>MSPLSGSLAPLNMKGLVKFQDVSFAYPNHPNVQVLQGLTFTLYPGKVTALVGPNGSGKSTVAALLQNLYQPTGGKVLLDGEPLVQYDHHYLHTQVAAVGQEPLL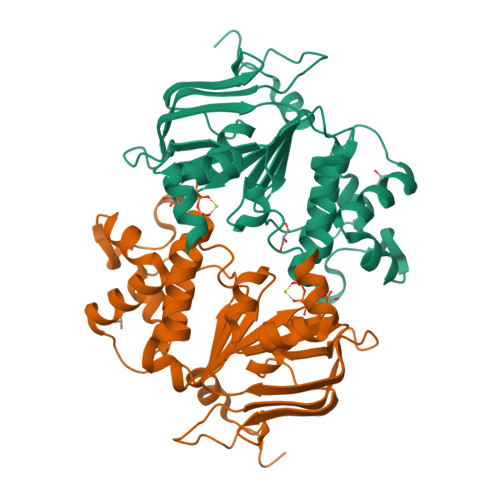FGRSFRENIAYGLTRTPTMEEITAVAMESGAHDFISGFPQGYDTEVGETGNQLSGGQRQAVALARALIRKPRLLILDQATSALDAGNQLRVQRLLYESPEWASRTVLLITHQLSLAERAHHILFLKEGSVCEQGTHLQLMERGGCYRSMVEALAAPSDAAAHHHHHH[4x]> QLLQPLPAEIKGTKLLAHWASGATITCIPESFLEDEQPIKKTLIKTIHGEKQQNVYYVTFKVKGRKVEAEVIASPYEYILLSPTDVPWLTQQPLQLTILVPLQEYQEKILSKTALPEDQKQQLKTLFVKYDNLWQHWENQVGHRKIRPHNIATGDYPPRPQKQYPINPKAKPSIQIVIDDLLKQGVLTPQNSTMNTPVYPVPKPDGRWRMVLDYREVNKTIPLTAAQNQHSAGILATIVRQKYKTTLDLANGFWAHPITPESYWLTAFTWQGKQYCWTRLPQGFLNSPALFTADVVDLLKEIPNVQVYVDDIYLSHDDPKEHVQQLEKVFQILLQAGYVVSL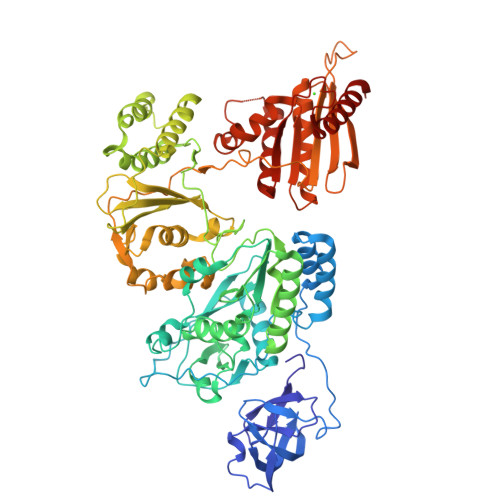KKSEIGQKTVEFLGFNITKEGRGLTDTFKTKLLNITPPKDLKQLQSILGLLNFARNFIPNFAELVQPLYNLIASAKGKYIEWSEENTKQLNMVIEALNTASNLEERLPEQRLVIKVNTSPSAGYVRYYNETGKKPIMYLNYVFSKAELKFSMLEKLLTTMHKALIKAMDLAMGQEILVYSPIVSMTKIQKTPLPERKALPIRWITWMTYLEDPRIQFHYDKTLPELKHIPDVYTSSQSPVKHPSQYEGVFYTDGSAIKSPDPTKSNNAGMGIVHATYKPEYQVLNQWSIPLGNHTAQMAEIAAVEFACKKALKIPGPVLVITDSFYVAESANKELPYWKSNGFVNNKKKPLKHISKWKSIAECLSMKPDITIQHEKGHQPTNTSIHTEGNALADKLATQGSYVVN>[3x]MANPVHKITDEKKQQGLEKINSGQRFKANLIKWVSFISGDMAAFGEWMKGQFILLQIMDWVLRGAAQVMFVNNPLSGLIIFAGLILQNRWWALNGFVGTVFATISALILCQNRGAIAAGLYGYNGILVGLLMAVFSNAGDWYWWLLLPNIFMSMACPIVSSALASINSRWDLPVFTLPFNILVCLHMVA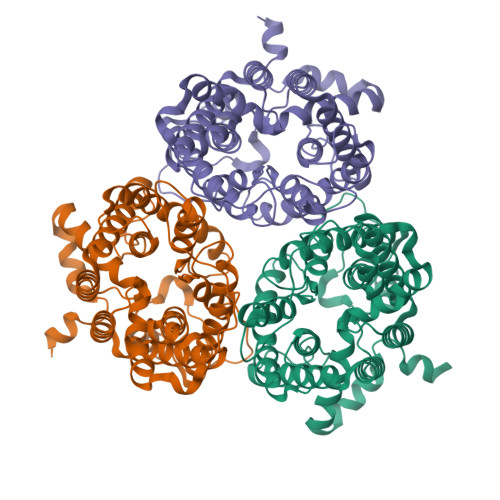TGHYNQYFPQILIQPTTSMSNLTWSELDYAQLFRSIPVGIGQVYGCDNAWTGGIFMIALFISSPITFAHATIGSAVGMVSGLALAAPFKNIYMGLWGYNCVLACIAIGGMFYALTWQTHLLAVACAFFCAYLGSAIGNVMSNFGLPACTWPFCLSALTFLLITTETKFIHKLPLAKVAYPEQNLRYYWKMKKEEKTQKGIQAKDTESQLEKEQISISMEKKDLDICTVDVQQEENTL>MAEKRTGLAEDGAKSVYERLKNDRAPYETRAQNCAQYTIPSLFPKDSDNASTDYQTPWQAVGARGLNNLASKLMLALFPMQTWMRLTISEYEAKQLLSDPDGLAKVDEGLSMVERIIMNYIESNSYRVTLFEALKQLVVAGNVLLYLPEPEGSNYNPMKLYRLSSYVVQRDAFGNVLQMVTRDQIAFGALPEDIRKAVEGQGGEKKADETIDVYTHIYLDEDSGEYLRYEEVEGMEVQGSDGTYPKEACPYIPIRMVRLDGESYGRSYIEEYLGDLRSLENLQEAIVKMSMISSKVIGLVNPAGITQPRRLTKAQTGDFVTGRPEDISFLQLEKQADFTVAKAVSDAIEARLSFAFMLNSAVQRTGERVTAEEIRYVASELEDTLGGVYSILSQELQLPLVRVLLKQLQATQQIPELPKEAVEPTISTGLEAIGRGQDLDKLERCVTAWAALAPMRDDPDINLAMIKLRIANAIGIDTSGILLTEEQKQQKMAQQSMQMGMDNGAAALAQGMAAQATASPEAMAAAADSVGLQPGI[12x]

Escherichia coli bacteriophage T7, a member of Podoviridae, has been used as a model for understanding the DNA packaging mechanism common to tailed phages and related dsDNA viruses. The phages package genomic dsDNA into a round procapsid using the portal in complex with an ATP-dependent terminase complex as the motor. At the beginning of phage infection, the tail is responsible for receptor recognition, and the portal and tail act as a tunnel for DNA delivery into the host cytoplasm. Here, we determined structures of the DNA packaging intermediate and mature capsids of T7 using cryo-electron microscopy (cryo-EM) and symmetry-mismatch reconstruction.

The DNA-free T7 capsid II particles, which were considered to be a DNA packaging intermediate subsequent to the T7 procapsid and morphogenetic precursor of the mature phage, were purified from cells for cryo-EM structural analysis. The local refinement and reconstruction improved the structural resolution of the portal to 4.9 Å. The lower resolution of the portal structure in the capsid II suggests that the portal might be flexible to some extent or deviate from 12-fold symmetry during the DNA packaging. The portal in the capsid II is formed by 12 copies of symmetrically arranged protein gp8 with similar topology but different conformation compared with the portal in the mature phage (discussed below). The absence of the barrel in our capsid II portal structure and in the phage procapsid portal structures suggests that the barrel is not involved in the DNA packaging. The portal clip region interacts with the rim of the open icosahedral vertex and five protrusions around the inner capsid surface. A structural comparison between the portal in the capsid II and that in the mature phage revealed that the portal undergoes considerable conformational changes from the packaging intermediate to the mature state. The whole portal moves downward, resulting in the exposure of the clip. This movement causes a squeeze between the inner capsid shell and the wing. Therefore, the wing undergoes a rigid-body rotation by approximately 25°.>MICLGLEGTAEK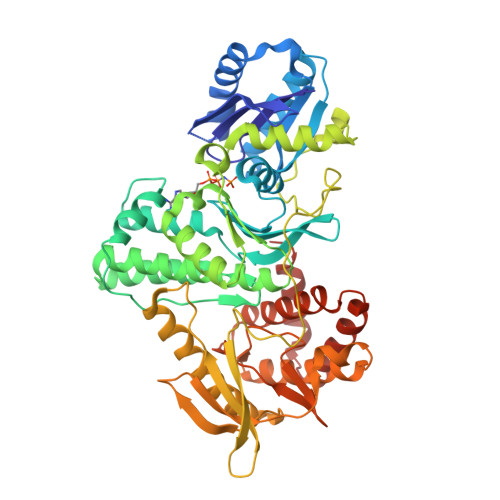TGVGIVTSDGEVLFNKTIMYKPPKQGINPREAADHHAETFPKLIKEAFEVVDKNEIDLIAFSQGPGLGPSLRVTATVARTLSLTLKKPIIGVNHCIAHIEIGKLTTEAEDPLTLYVSGGNTQVIAYVSKKYRVFGETLDIAVGNCLDQFARYVNLPHPGGPYIEELARKGKKLVDLPYTVKGMDIAFSGLLTAAMRAYDAGERLEDICYSLQEYAFSMLTEITERALAHTNKGEVMLVGGVAANNRLREMLKAMCEGQNVDFYVPPKEFCGDNGAMIAWLGLLMHKNGRWMSLDETKIIPNYRTDMVEVNWIKEIKGKKRKIPEHLIGKGAEADIKRDSYLDFDVIIKERVKKGYRDERLDENIRKSRTAREARYLALVKDFGIPAPYIFDVDLDNKRIMMSYINGKLAKDVIEDNLDIAYKIGEIVGKLHKNDVIHNDLTTSNFIFDKDLYIIDFGLGKISNLDEDKAVDLIVFKKAVLSTHHEKFDEIWERFLEGYKSVYDRWEIILELMKDVERRARYVE[2x]(1R)-2-[(2S)-2-methyl-3-sulfanyl-propanoyl]-3,4-dihydro-1H-isoquinoline-1-carboxylic 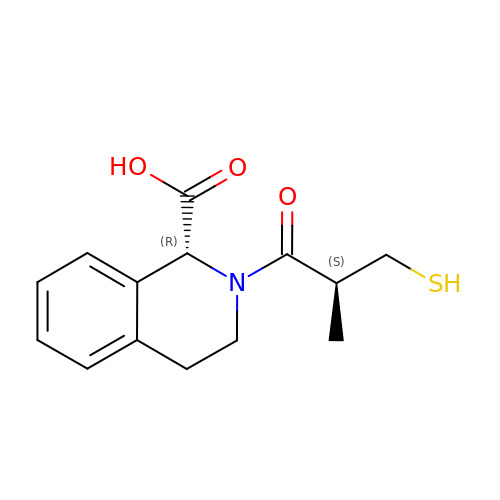acid | C14 H17 N O3 S | DMGKNMLYAQKRNE-BXKDBHETSA-N>[2x]LVPRGSDSSRRQYQEKYKQVEQYMSFHKLPADFRQKIHDYYEHRYQGKMFDEDSILGELNGPLREEI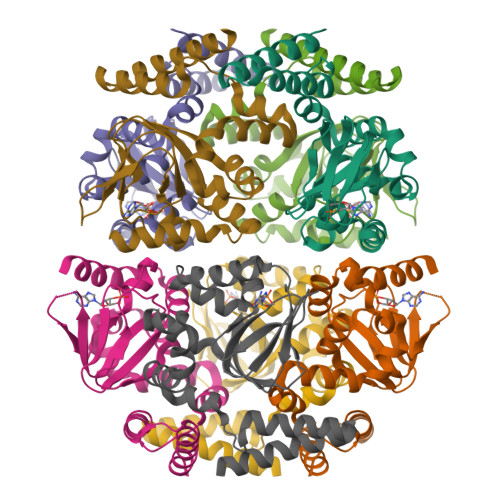VNFNNRKLVASMPLFANADPNFVTAMLTKLKFEVFQPGDYIIREGTIGKKMYFIQHGVVSVLTKGNKEMKLSDGSYFGEISLLTRGRRTASVRADTYSRLYSLSVDNFNEVLEEYPMMRRAFETVAIDRLDRIGKKN>[4x]GKKKGPKYDQIIDAAVQVIAEHGYHQAQVSKIAKAAGVADGTIYLYFNNKEDVLISLFQEKMG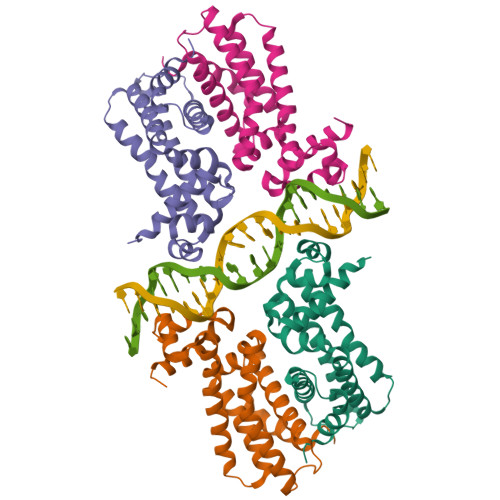RFVDKIRSQMNEATDVEEKLKILVNMHFKQLAADHKLAIVTQLELRQSNTELRLKINEVLKGYLNLLDELLMEGKEKGYFFQELDTRLARQMIFGTLDEVVTNWVMKDCKYDLTALVKPVHQLLLGGLRHR> MYQKVNCYSILFLKGVDKMKTQLNPFVVANPAKCIGCKACEVACFAVHNRNNHVGATVGTVSIPVIPRLHLIKTEHGTMPIQCRHCEDAPCANVCTVGAIKREGN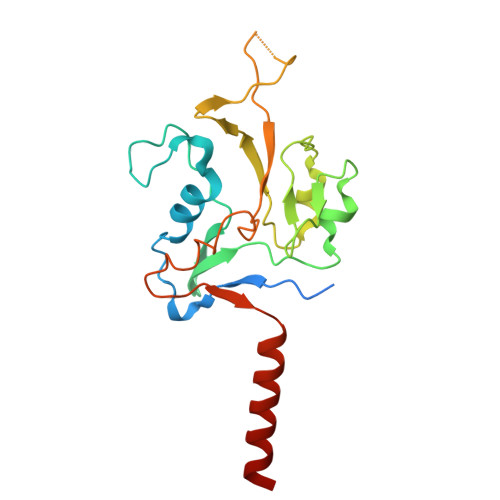AIVVDEKLCIGCKSCLLACPFGAIELLPQYEDGREVFQINLKEESESGLVQEPRIIAYKCDLCNDLGEPACVKACPENALTLVMPTEMKKARNKEAALSFLRVVR> SGGRNVTSIALRAETWLLAAWHVKVPPMWLEACINWIQEENNNVNLSQAQMNKQVFEQWLLTDLRDLEHPLLP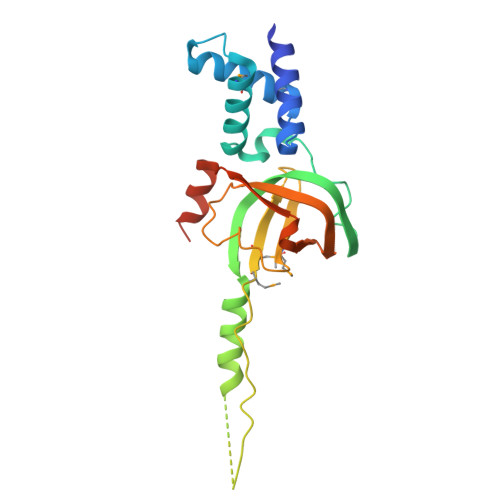DGILEIPKGELNGFYALQINSLVDVSQPAYSQIQKLRGKNTTNDLVTAEAQVTPKPWEAKPSRMLMLQLTDGIVQIQGMEYQPIPILHSDLPPGTKILIYGNISFRLGVLLLKPENVKVLGGEVDALLEEYAQEKVLARLIGE(3a,5a)-3-Hydroxypregnane-11,20-dione | C21 H32 O3 | 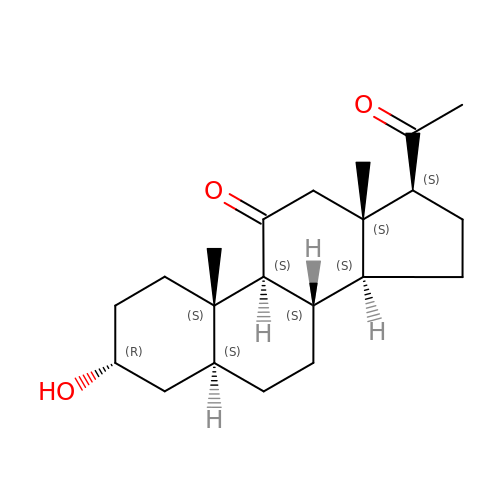DUHUCHOQIDJXAT-OLVMNOGESA-N>[8x]MSNRYQAKFAALKAQDKGAFVPFVTIGDPSPELSLKIIQTLVDNGADALELGFPFSDPLADGPVIQGANLRSLAAGTTSSDCFDIITKVRAQHPDM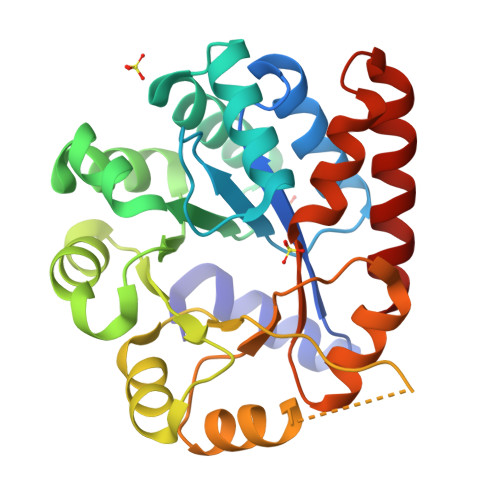PIGLLLYANLVFANGIDEFYTKAQAAGVDSVLIADVPVEESAPFSKAAKAHGIAPIFIAPPNADADTLKMVSEQGEGYTYLLSRAGVTGTESKAGEPIENILTQLAEFNAPPPLLGFGIAEPEQVRAAIKAGAAGAISGSAVVKIIEAHQHDEATLLAKLAEFTTAMKAAT>MARQVFDDKLLAVIS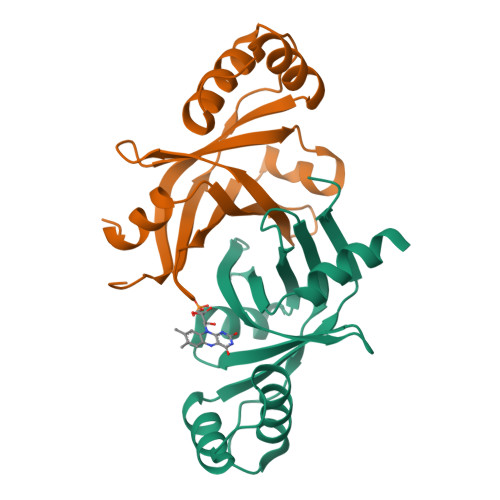GNSIGVLATIKHDGRPQLSNVQYHFDPRKLLIQVSIAEPRAKTRNLRRDPRASILVDADDGWSYAVAEGTAQLTPPAAAPDDDTVEALIALYRNIAGEHSDWDDYRQAMVTDRRVLLTLPISHVYGLPPGMR[2x]> MEEVKKDVYSVWALPDEESEPRFKKLMEALRSEFTGPRFVPHVTVAVSAYLTADEAKKMFESACDGLKAYTATVDRVSTGTFFFQCVFLLLQTTPEVMEAGEHCKNHFNCSTTTPYMPHLSLLYAELTEEEKKNAQEKAYTLDSSLDGLSFRLNRLALCKT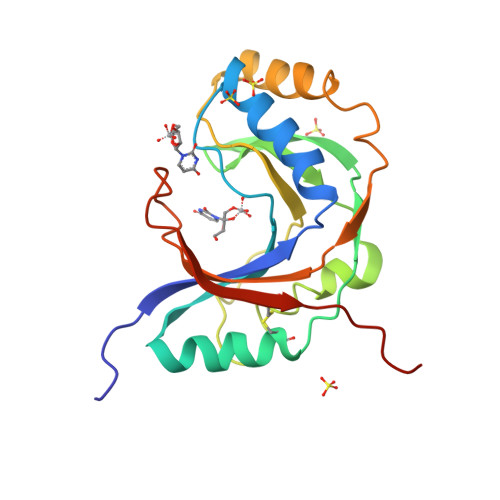DTEDKTLETWETVAVCNLNPGSHHHHHH>MMNVIMREIGKKLDELSREFYESVIPPIDMYEEGGELVVVADLAGFNKDKISVRLSAQNELIINAEREIQYIGTKYATQRPLKIHKVIRLPVKVKRDSQV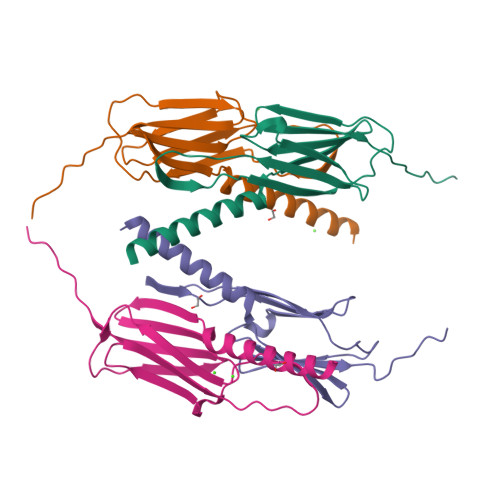TAKYENGVLTIRIPVEGSVSIRIE[4x]2-[[2,6-bis(chloranyl)-3-[(2,2-dimethylpropanoylamino)methyl]phenyl]amino]-1-methyl-6-(2-methyl-2-oxidanyl-propoxy)-N-[2,2,2-tris(fluoranyl)ethyl]benzimidazole-5-carboxamide 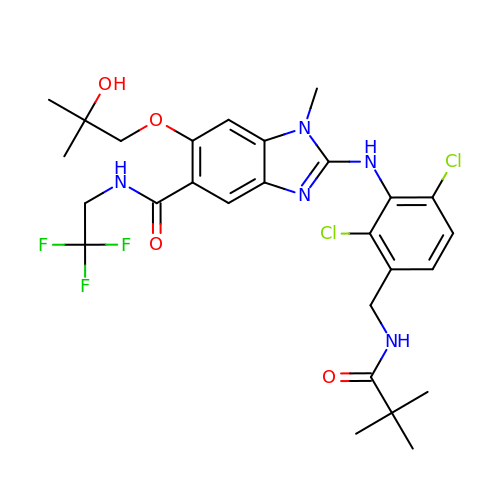| C27 H32 Cl2 F3 N5 O4 | CHFOASGROVVRSK-UHFFFAOYSA-N>[8x]SNATDGQLTKQHVRALAISALAPKPHETLWDIGGGSGSIAIEWLRSTPQTTAVCFEISEERRERILSNAINLGVSDRIAVQQGAPRAFDDVPDNPDVIFIGGGLTAPGVFA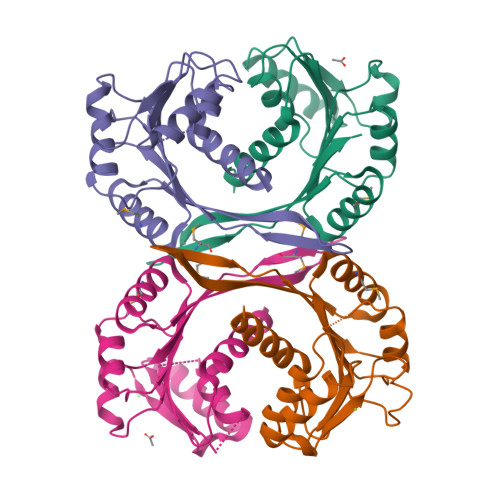AAWKRLPVGGRLVANAVTVESEQMLWALRKQFGGTISSFAISHEHTVGSFITMKPALPVHQWTVVKA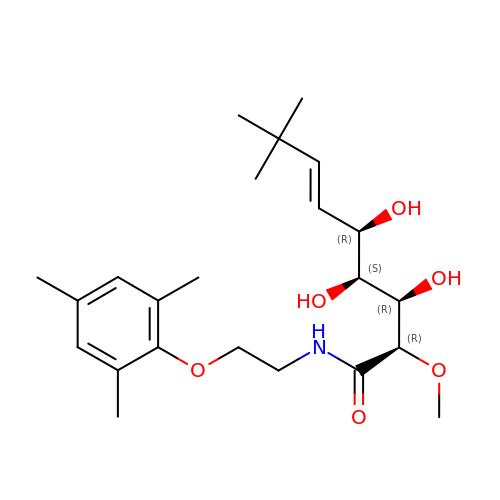(2R,3R,4S,5R,6E)-3,4,5-trihydroxy-2-methoxy-8,8-dimethyl-N-[2-(2,4,6-trimethylphenoxy)ethyl]non-6-enamide | C23 H37 N O6 | UMRMEUOEFMNZRM-SWQIVCBNSA-N>[6x]MRVVIQRVKGAILSVRKENIGENEKELEIISEIKNGLICFLGIHKNDTWEDALYIIRKCLNLRLWNNDNKTWDKNVKDLNYELLIVSQFTLFGNTKKGNKPDFHLAKEPNEALIFYNK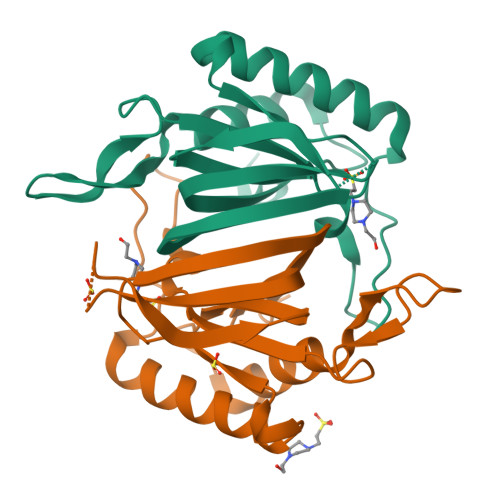IIDEFKKQYNDDKIKIGKFGNYMNIDVTNDGPVTIYIDTHDINLNK> MGSSHHHHHHSSGENLYFQGSHMMTDAKAFRRYIFELYFDPARLLELDDDQHLQRIERFLDALAPLHPVLENWYLCGDSLRDALSHNVTEHRQDLAKALSRDRRTRAVELVLWNGEEDPLKGGLSLDYEASGRAVSSRLQLEDAGSLLQVFDAPASSFVAIFL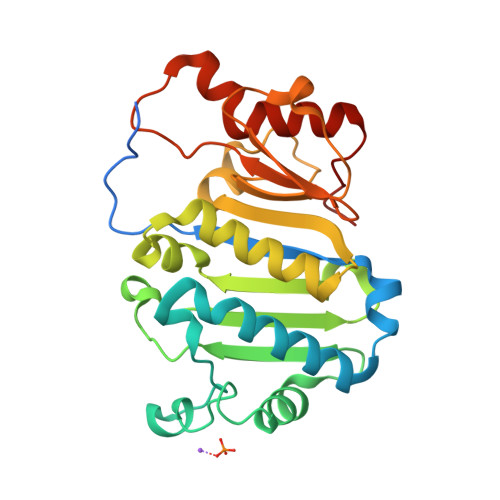AVLEIWPETTWGMLAPHAYFVHQRTFPDRRSIGWIGFCPHPLRATDFPAATELVDIPGRGTLLLNGREPMDETRREHFERVGEADIKLMELGYLPPLRG> MQKHWWHKATVYQIYPKSFMDTNGDGIGDLKGITSKLDYLQKLGVMAIWLSPVYDSPMDDNGYDIANYEAIADIFGNMADMDNLLTQAKMRGIKIIMDLVVNHTSDEHAWFIEAREHPDSSERDYYIWCDQPNDLESIFGGSAWQYDDKSDQYYLHFFSKKQPDLNWENANLRQKIYDMMNFWIDKGIGGFRMDVIDMIGKIPAQHIVSNGPKLHAYLKEMNAASFGQHDLLTVGETWGATPEIAKQYSNPVNHELSMVFQFEHIGLQHKPEAPKWDYVKELNVPALKTIFNKWQTELELGQGWNSLFWNNHDLPRVLSIWGNTGKYREKSAKALAILLHLMRGTPYIYQGEEIGMTNYPFKDLNELDDIESLNYAKEAFTNGKSMETIMDSIRMIGRDNARTPMQWDASQNAGFSTADKTWLPVNPNYKDINVQAALKNSNSIFYTYQQLIQLRKENDWLVDADFELLPTADKVFAYLRKVREERYLIVVNVSDQEEVL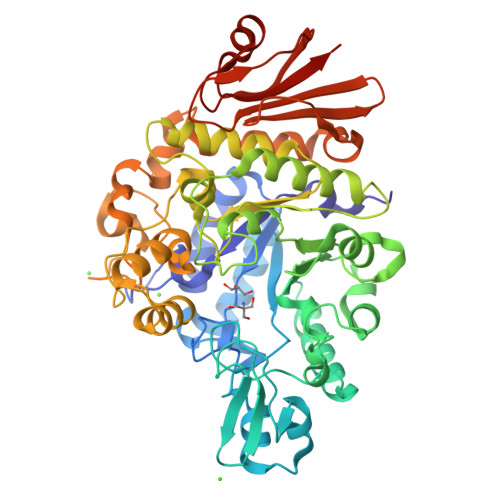EIDVDKQETLISNTNESAALANHKLQPWDAFCIKILEHHHHHH~{N}-[(4~{S},5~{S})-2-[2-(1~{H}-imidazol-4-yl)ethyl]-5-methyl-3-oxidanylidene-1,2-oxazolidin-4-yl]-2,3-bis(oxidanyl)benzamide | C16 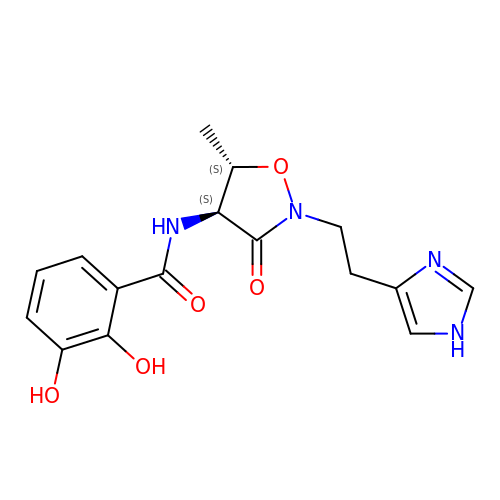H18 N4 O5 | YQXURFXJBIFMOA-ZANVPECISA-N> MRVNNGLTPQELEAYGISDVHDIVYNPSYDLLYQEELDPSLTGYERGVLTNLGAVAVDTGIFTGRSPKDKYIVRDDTTRDTFWWADKGKGKNDNKPLSPET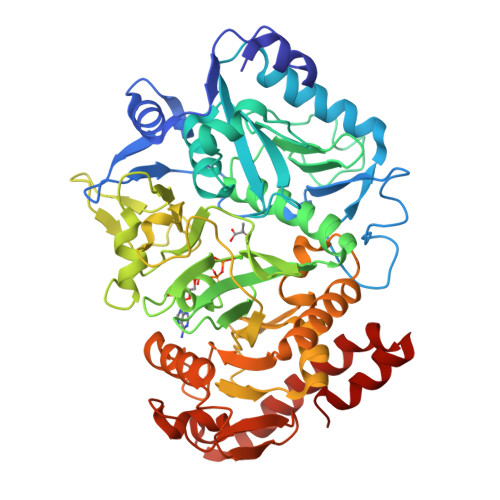WQHLKGLVTRQLSGKRLFVVDAFCGANPDTRLSVRFITEVAWQAHFVKNMFIRPSDEELAGFKPDFIVMNGAKCTNPQWKEQGLNSENFVAFNLTERMQLIGGTWYGGEMKKGMFSMMNYLLPLKGIASMHCSANVGEKGDVAVFFGLSGTGKTTLSTDPKRRLIGDNEHGWDDDGVFNFEGGCYAKTIKLSKEAEPEIYNAIRRDALLENVTVREDGTIDFDDGSKTENTRVSYPIYHIDNIVKPVSKAGHATKVIFLTADAFGVLPPVSRLTADQTQYHFLSGFTAKLAGTERGITEPTPTFSACFGAAFLSLHPTQYAEVLVKRMQAAGAQAYLVNTGWNGTGKRISIKDTRAIIDAILNGSLDNAETFTLPMFNLAIPTELPGVDTKILDPRNTYASPEQWQEKAETLAKLFIDNFDKYTDTPAGAALVAAGPKL> IEMKPHPWFFGKIPRAKAEEMLSKQRHDGAFLIRESESAPGDFSLSVKFGNDVQHFKVLRDGAGKYFLWVVKFN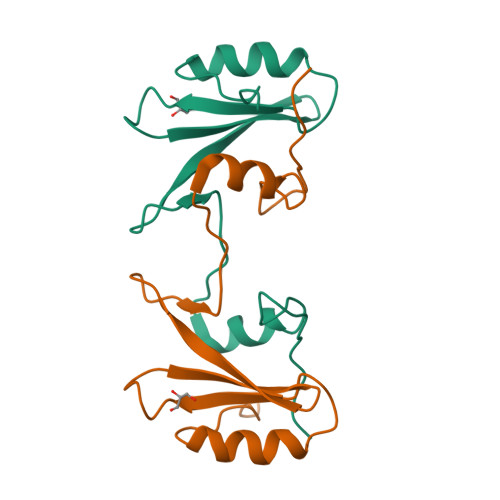SLNELVDYHRSTSVSRNQQIFLRDIEQVPQQPTYVQHHHHHH>[2x]KEE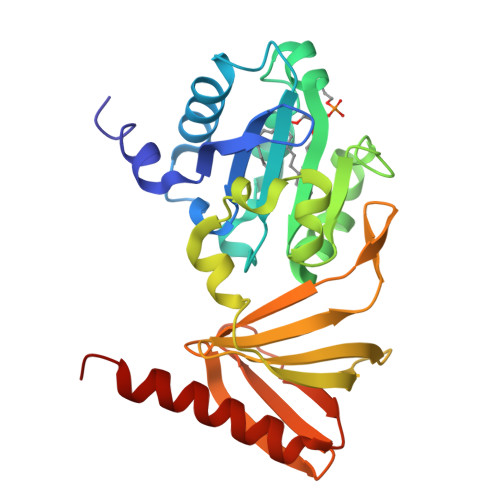FKALKTLSIFYQAGTSKAGNPIFYYVARRFKTGQINGDLLIYHVLLTLKPYYAKPYEIVVDLTHTGPSNRFKTDFLSKWFVVFPGFAYDNVSAVYIYNCNSWVREYTKYHERLLTGLKGSKRLVFIDCPGKLAEHIEHEQQKLPAATLALEEDLKVFHNALKLAHKDTKVSIKVGSTAVQVTSAERTVLGQSVFLNDIYYASEIEEICLVDENQFTLTIANQGTPLTFMHQECEAIVQSIIHIRTRWELSQPD> APLVHHHHHHALDENLYFQGALADVSRPPHARKTGGSSPETKYDQPPKCDISGKEAISALSRAKSKHCRQEIGETYCRHKLGLLMPEKVTRFCPLEGKANKNVQWDEDSVEYMPANPVRIAFVLVVHGRASRQLQRMFKAIYHKDHFYYIHVDKRSNYLHRQVLQVSRQYSNVRVTPWRMATIWGGASLLSTYLQSMRDLLEMTDWPWDFFINLSAADYPIRTNDQLVAFLSRYRDMNFLKSHGRDNARFIRKQGLDRLFLECDAHMWRLGDRRIPEGIAVDGGSDWFLLNRRFVEYVTFSTDDLVTKMKQFYSYTLLPAESFFHTVLENSPHCDTMVDNNLRITNWNRKLGCKCQYKHIVDWCGCSPNDFKPQDFHRFQQTARPTFFARKFEAVVNQEIIGQLDYYLYGNYPAGTPGLRSYWENVYDEPDGIHSLSDVTLTLYHSFARLGLRRAETSLHTDGENSCRYYPMGHPASVHLYFLADRFQGFLIKHHATNLAVSKLETLETWVMPKKVFKIASPPSDFGRLQFSEVGTDWDAKERLFRNFGGLLGPMDEPVGMQKWGKGPNVTVTVIWVDPVNVIAATYDIL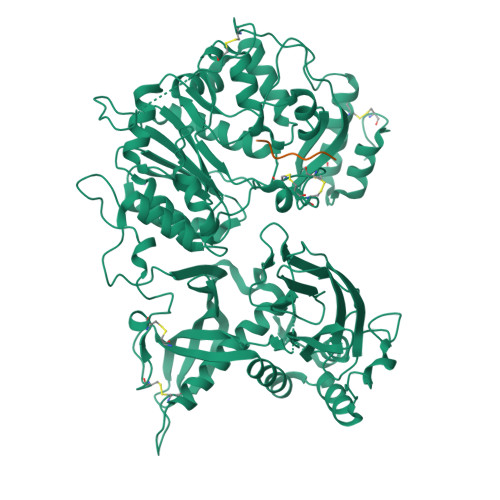IESTAEFTHYKPPLNLPLRPGVWTVKILHHWVPVAETKFLVAPLTFSNRQPIKPEEALKLHNGPLRNAYMEQSFQSLNPVLSLPINPAQVEQARRNAASTGTALEGWLDSLVGGMWTAMDICATGPTACPVMQTCSQTAWSSFSPDPKSELGAVKPDGRLR;> QEEEYSGGGQGG>[4x]APITAPDITSICKDASSGIGNQEGAIRTRKCCPPSLGKKIKDFQFPNDKKVRMRWPAHKGTKKQVDDYRRAIAAMRALPDDDPRSFVSQAKIHCAYCNGGYTQVDSGFPDIDI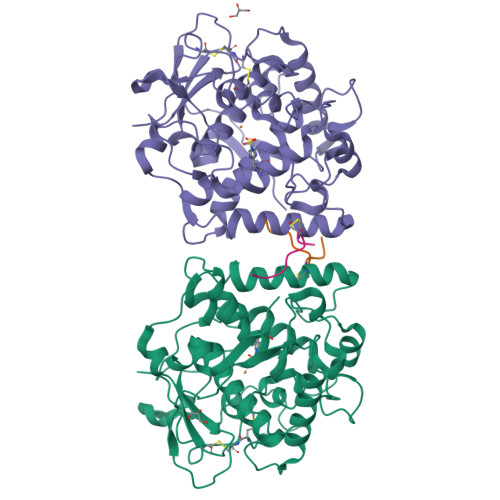QIHNSWLFFPFHRWYLYFYERILGSLIDEPNFALPYWKWDEPKGMPISNIFLGDASNPLYDQYRDANHIEDRIVDLDYDGKDKDIPDQQQVACNLSTVYRDLVRNGVDPTSFFGGKYVAGDSPVANGDPSVGSVEAGSHTAVHRWVGDPTQPNNEDMGNFYSAGYDPVFYIHHANVDRMWKLWKELRLPGHVDITDPDWLNASYVFYDENKDLVRVYNKDCVNLDKLKYNFIENSKE;>DGVFTTPCDPEYAGG[4x]> MSNPIRDIQDRLKTAKFDNKDDMMNLASSLYKYEKQLMDSSEATLCQQGLSNRPNSFSQLSQFRDSDIQSKAGGQTGKFWQNEYEACKNFQTHKERRETLEQIIRFLQNGAEEKDADDLLLKTLARAYFHRGLLYRPKGFSVPARKVEAMKKAIAYCEIILDKNEEESEALRIWLYAAMELRRCGEEYPENFAEKLFYLANDGFISELYDIRLFLE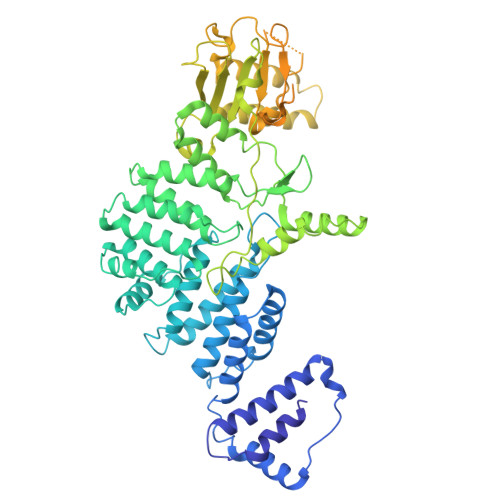YTEREEDNNFLDMILQENQDRERLFELCLYKARACFHLNQLNDVRIYGESAIDNAPGAFADPFWDELVEFIRMLRNKKSELWKEIAIKAWDKCREKEMKVGNNIYLSWYWARQRELYDLAFMAQDGIEKKTRIADSLKSRTTLRIQELNELRKDAHRKQNRRLEDKLDRIIEQENEARDGAYLRRNPPCFTGGKREEIPFARLPQNWIAVHFYLNELESHEGGKGGHALIYDPQKAEKDQWQDKSFDYKELHRKFLEWQENYILNEEGSADFLVTLCREIEKAMPFLFKSEVIPEDRPVLWIPHGFLHRLPLHAAMKSGNNSNIEIFWERHASRYLPAWHLFDPAPYSREESSTLLKNFEEYDFQNLENGEIEVYAPSSPKKVKEAIRENPAILLLLCHGEADMTNPFRSCLKLKNKDMTIFDLLTVEDVRLSGSRILLGACESDMVPPLEFSVDEHLSVSGAFLSHKAGEIVAGLWTVDSEKVDECYSYLVEEKDFLRNLQEWQMAETENFRSENDSSLFYKIAPFRIIGFPAE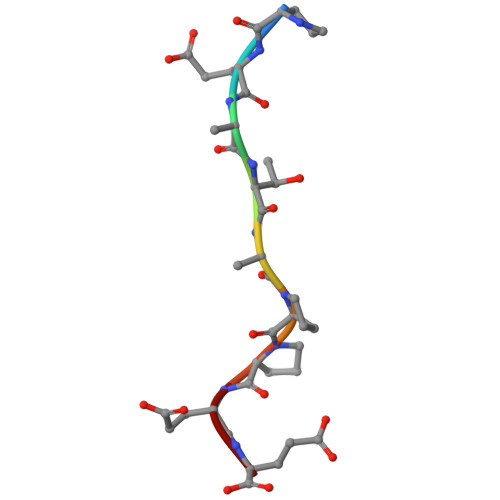> PEATAPPEE>MGSITENTSWNKEFSAEAVNGVFVLCKSSSKSCATNDLARASKEYLPASTFKIPNAIIGLETGVIKNEHQVFKWDGKPRAMKQWERDLTLRGAIQVSAVPVFQQIAREVGEVRMQKYLKKFSYGNQNISGGIDKFGLEGQLRISA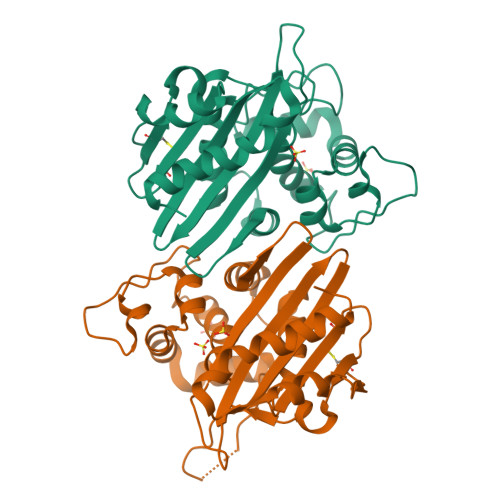VNQVEFLESLYLNKLSASKENQLIVKEALVTEAAPEYLVHSKTGFSGVGTESNPGVAWWVGWVEKETEVYFFAFNMDIDNESKLPLRKSIPTKIMESEGIIGG[4x]5-[4-methoxy-3-[4-[4-(1~{H}-1,2,3,4-tetrazol-5-yl)phenoxy]butoxy]phenyl]-4,4-dimethyl-2-propan-2-yl-pyrazol-3-one | C26 H32 N6 O4 | 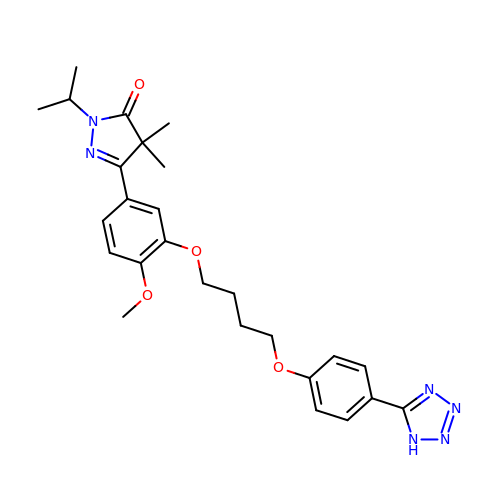LSMMVMRAIOYJHV-UHFFFAOYSA-N> TGGRSMSDSQIVTPGELVTDDPIWMRGHGTYFLDNMTYSSVAGTVSRVNRLLSVIPLKGRYAPETGDHVVGRIAEVGNKRWKVDIGGKQHAVLMLGSVNLPGGILRRKSESDELQMRSFLKEGDLLNAEVQSLFQDGSASLHTRSLKYGKLRNGMFCQVPSSLIVRAKNHTHNLPGNITVVLGVNGYIWLRKTSQMDLARDTPSANNSSSIKSTGPTGAVSLNPSITRLEEESSWQIYSDENDPSISNNIRQAICRYANVIKALAFCEIGITQQRIV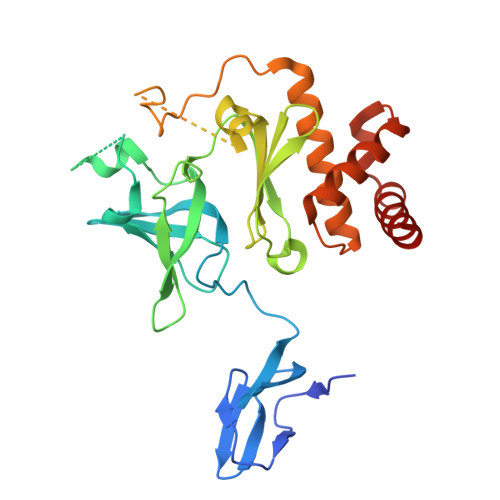SAYEASMVYSNVGELIEKNVMESIGSDILTAEKMRGNGN>[16x]MGARNSVLRGKKADELEKV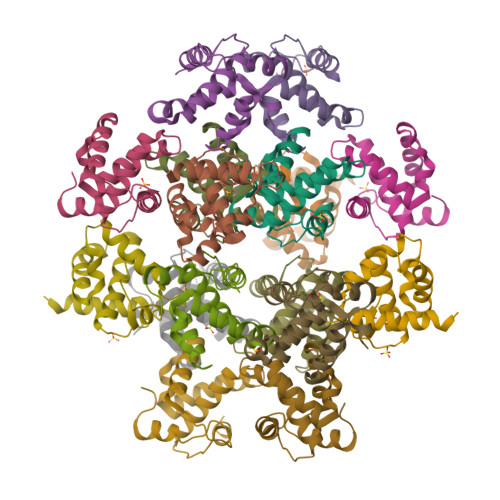RLRPGGKKKYRLKHIVWAANELDKFGLAESLLESKEGCQKILRVLDPLVPTGSENLKSLFNTVCVIWCLHAEEKVKDTEEAKKLAQRHLVAETGTAEKMPNTSRPTAPPSGKRGNY> MADADVQPAGSVPIPDGPAQTWIVADLDSGQVLAGRDQNVAHPPASTIKVLLALVALDELDLNSTVVADVADTQAECNCVGVKPGRSYTVRQLLDGLLLVSGNDAANTLAHMLGGQDVTVAKMNAKAATLGATSTHATTPSGLDGPGGSGASTAHDLVVIFRAAMANPVFAQIIAEPSAMFPSDDGEQLIVNQDELLQRYPGAIGGKTGYTNAARKTFVGAAARGGRRLVIAMMYGLVKEGGPTYWDQAATLFDWGFALNPQASVDSLGSHHHHHH

Here, we presented structural and phylogenetic analyses of two meropenem-sensitive Mtb penicillin-binding proteins, Rv2911 and Rv3330. A search of the Mtb genome for Peptidase_S11 Pfam family proteins (PF00768) yielded two hits: Rv2911 and Rv3330. The active sites of both proteins contain the three typical penicillin-binding protein motifs: SXXK, SXN, and KTG. The structures showed similar overall folds containing two subdomains.

Because the wild-type Rv2911 was poorly soluble and failed to crystallize, we undertook extensive construct optimization using the GFP folding reporter method. Several rounds of directed evolution to improve solubility yielded an optimized gene sequence carrying six point mutations. The resulting A113V, T197I, N208D, G289D quadruple-mutant protein was named Rv2911opt. The Rv2911opt-PMSF structure was determined at 2.0 Å resolution using multiwavelength anomalous dispersion of Se-labeled enzyme. Rv2911opt was bound to a molecule of the nonspecific inhibitor, PMSF, carried over from the purification. In both structures, the inhibitors were covalently linked to the serine of the first motif (STIK in Rv2911, SVIK in Rv3330). In the Rv2911opt-PMSF structure the conformation of the inhibitor was not unique, and the electron density for the phenyl group of the ligand suggested at least two alternate conformations. Neither conformation appeared stabilized by additional enzyme-inhibitor interactions. Cys100 of Rv2911opt was found in a disulfide with Cys102 from a symmetry-related molecule. In the Rv3330 crystals, Cys77 residues from adjacent molecules formed a disulfide across a two-fold axis. Of the four mutations in Rv2911opt, two, A113V and T197I, were buried, while the other two, N208D and G289D, were exposed and participated in a crystal contacts.Simvastatin acid | C25 H40 O6 | 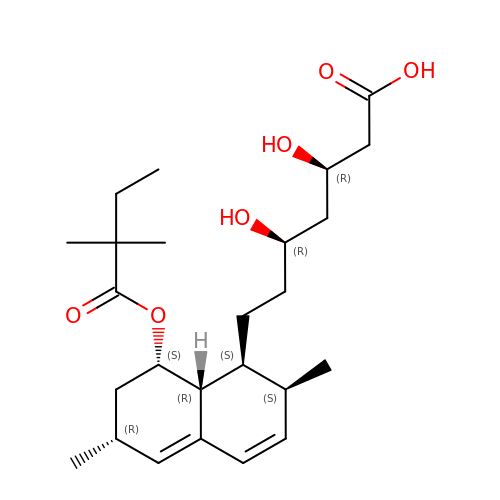XWLXKKNPFMNSFA-HGQWONQESA-N PURINE RIBOSIDE-5'-MONOPHOSPHATE | C10 H13 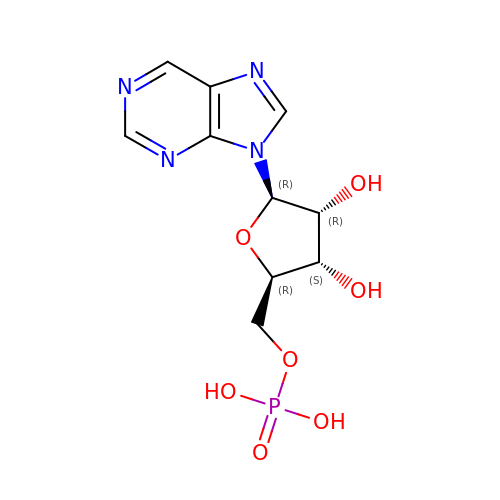N4 O7 P | MCWDCZIDTUQRHK-FDDDBJFASA-N>ALKTLNLGSCVIATNLQEIRNGFSEIRGSVQAKDGNIDIRILRRTESLQDTKPANRCCLLRHLLRLY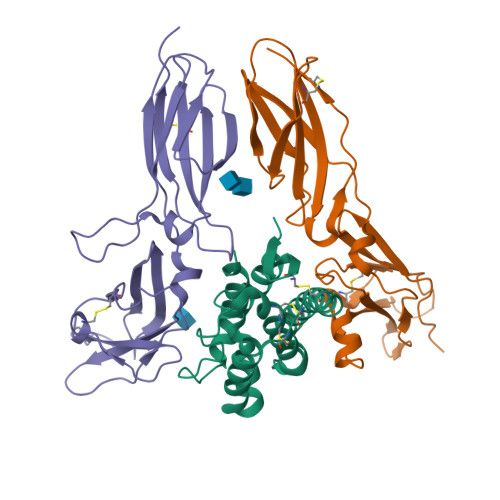LDRVFKNYQTPDHYTLRKISSLANSFLTIKKDLRLCHAHMTCHCGEEAMKKYSQILSHFEKLEPQAAVVKALGELDILLQWMEETE[2x];>ADEVAILPAPQQLSVLSTNMKHLLMWSPVIAPGETVYYSVEYQGEYESLYTSHIWIPSSWCSLTEGPECDVTDDITATVPYNLRVRATLGSQTSAWSILKHPFNRQSTILTRPGMEITKDGFHLVIELEDLGPQFEFLVAYWRREPGAEEHVKMVRSGGIPVHLETMEPGAAYCVKAQTFVKAIGRYSAFSQTECVEVQGEAIEGR[2x];>[2x]AVPCVSGGLPKPANITFLSINMKNVLQWTPPEGLQGVKVTYTVQYFIYGQKKWLNKSECRNINRTYCDLSAETSDYEHQYYARVRAIWGTKCSKWAESGRFYPFLETQIGPPEVALTTDEKSISVVLTAPEKWKRNPEDLPVSMQQIYSNLKYNVSVLNTKSNRTWSQCVTNHTLVLTWLEPNTLYCVHVESFVPGPPRRAQPSEKQCARTLKDQSSIEGR(5S)-5-(3-AMINOPROPYL)-3-(2,5-DIFLUOROPHENYL)-N-ETHYL-5-PHENYL-4,5-DIHYDRO-1H-PYRAZOLE-1-CARBOXAMIDE | C21 H24 F2 N4 O | 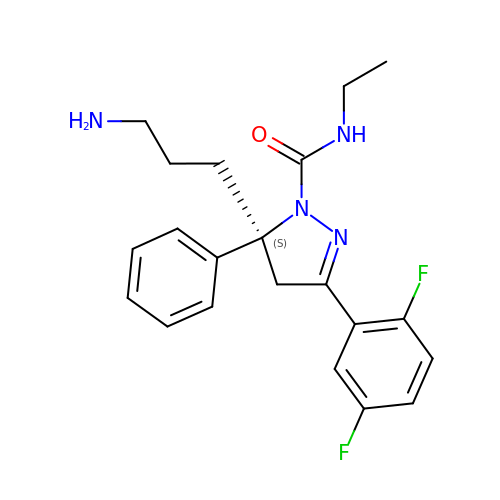OQMVLDZJPRSNOG-NRFANRHFSA-N> CCTGA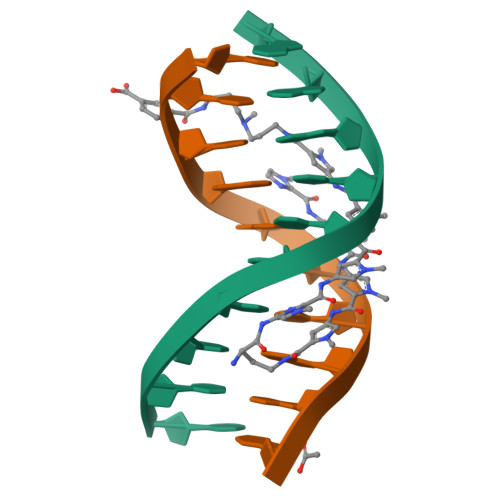CCAGG;> CCTGGTCAGG5-S-methyl-5-thio-alpha-D-ribofuranose | C6 H12 O4 S | 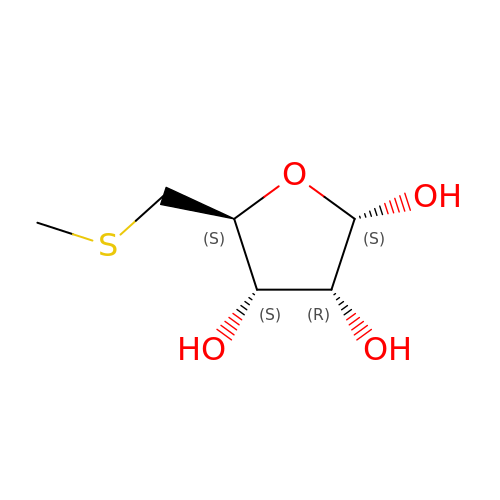OLVVOVIFTBSBBH-KAZBKCHUSA-N> VIPDYFKQSFPEGYSWERSMTYEDGGICIATNDITMEGDSFINKIHFKGTNFPPNGP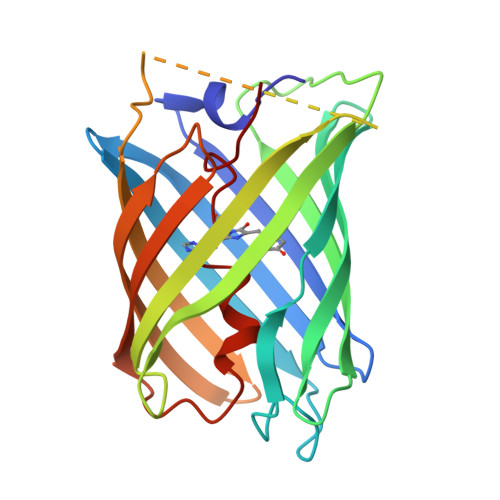VMQKRTVGWEASTEKMYERDGVLKGDVKMKLLLKGGGHYRCDYRTTYKVKQKPVKLPDYHFVDHRIEILSHDKDYNKVKLYEHAVARNSTDSMDELYKGGSGGMVSKGEETITSVIKPDMKNKLRMEGNVNGHAFVIEGEGSGKPFEGIQTIDLEVKEGAPLPFAYDILTTAFHYGNRVFTKYPR>[7x]MIVTPASIKALMTSWRKDFQGGLEDAPSQYNKIAMVVNSSTRS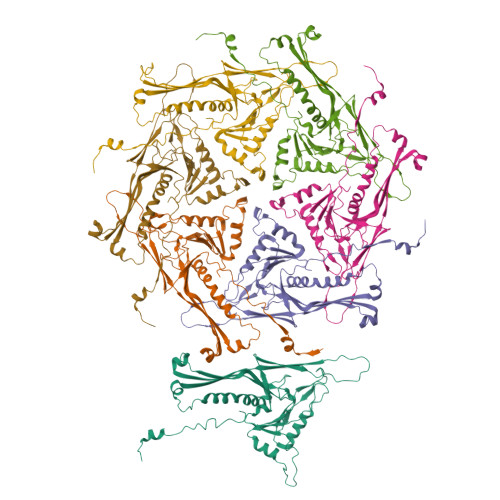NTYGWLGKFPTLKEWVGKRTIQQMEAHGYSIANKTFEGTVGISRDDFEDDNLGIYAPIFQEMGRSAAVQPDELIFKLLKDGFTQPCYDGQNFFDKEHPVYPNVDGTGSAVNTSNIVEQDSFSGLPFYLLDCSRAVKPLIFQERRKPELVARTRIDDDHVFMDNEFLFGASTRRAAGYGFWQMAVAVKGDLTLDNLWKGWQLMRSFEGDGGKKLGLKPTHIVVPVGLEKAAEQLLNRELFADGNTTVSNEMKGKLQLVVADYL>YY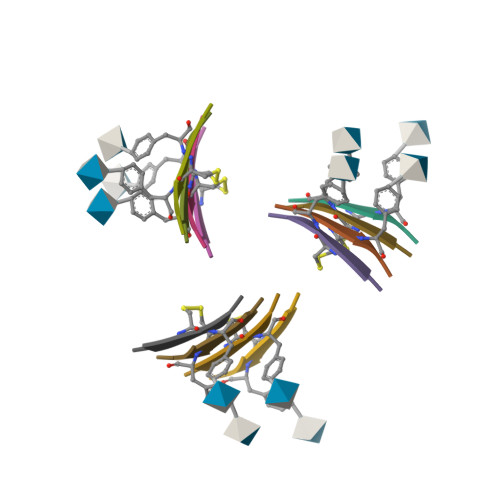CYY[12x]> SLGIFPT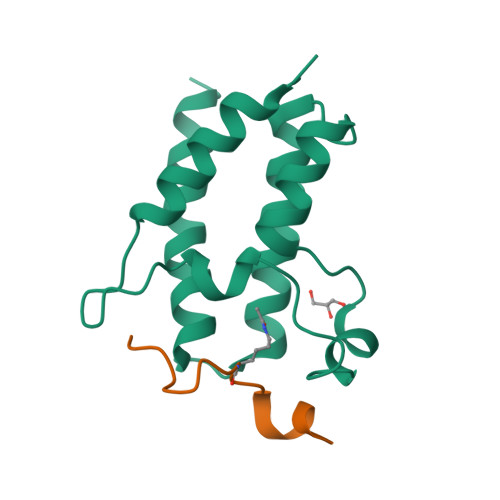VEKLVEEMREQLDEVDSHPRTSIFEKLPSKRDYPDYFKVIEKPMAIDIILKNCKNGTYKTLEEVRQALQTMFENARFYNEEGSWVYVDADKLNEFTDEWFKEHSS;> TARKSTGGKAPRKQLAY>KHLPEPFRIRVIEPVKRTTRAYREEAIIKSGMNPFLLDSEDVFIDLLTDSGTGAVTQSMQAAMMRGDEAYSGSRSYYAL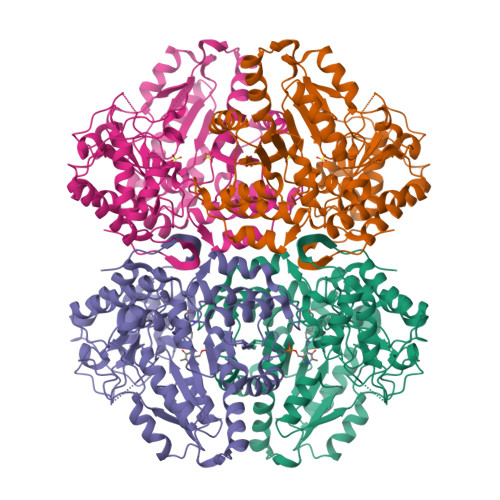AESVKNIFGYQYTIPTHQGRGAEQIYIPVLIKKREQEKGLDRSKMVAFSNYFFDTTQGHSQINGCTVRNVYIKEAFDTGVRYDFKGNFDLEGLERGIEEVGPNNVPYIVATITSNSAGGQPVSLANLKAMYSIAKKYDIPVVMDSARFAENAYFIKQREAEYKDWTIEQITRETYKYADMLAMSAKKDAMVPMGGLLCMKDDSFFDVYTECRTLCVVQEGFPTYGGLEGGAMERLAVGLYDGMNLDWLAYRIAQVQYLVDGLEEIGVVCQQAGGHAAFVDAGKLLPHIPADQFPAQALACELYKVAGIRAVEIGSFLLGRDPKTGKQLPCPAELLRLTIPRATYTQTHMDFIIEAFKHVKENAANIKGLTFTYEPKVLRHFTAKLKEV[2x]>[2x]PSVYDAAAQLTADVKKDLR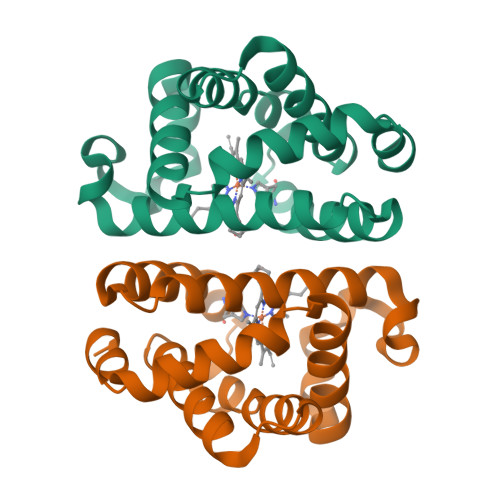DSWKVIGSDKKGNGVALATTLFADNQETIGYFKRLGDVSQGMANDKLRGHSITLMYALQNFIDQLDNPDDLVCVVEKFAVNHITRKISAAEFGKINGPIKKVLASKNFGDKYANAWAKLVAVVQAAL>[2x]MHHHHHHGSENLYFQGSMPEESS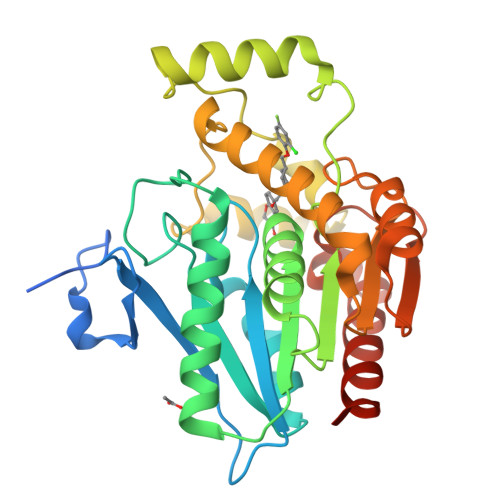PRRTPQSIPYQDLPHLVNADGQYLFCRYWAPTGTPKALIFVSHGAGEHSGRYEELARMLMGLDLLVFAHDHVGHGQSEGERMVVSDFHVFVRDVLQHVDSMQKDYPGLPVFLLGHSMGGAIAILTAAERPGHFAGMVLISPLVLANPESATTFKVLAAKVLNSVLPNLSSGPIDSSVLSRNKTEVDIYNSDPLICRAGLKVCFGIQLLNAVSRVERALPKLTVPFLLLQGSADRLCDSKGAYLLMELAKSQDKTLKIYEGAYHVLHKELPEVTNSVFHEINMWVSQRTATAGTASPP>[2x]MSFTPANRAYPYTRLRRNRRDDFSRRLVRENVLTVDDLILPVFVLDGVNQRESIPSMPGVERLSIDQLLIEAEEWVALGIPALALFPVT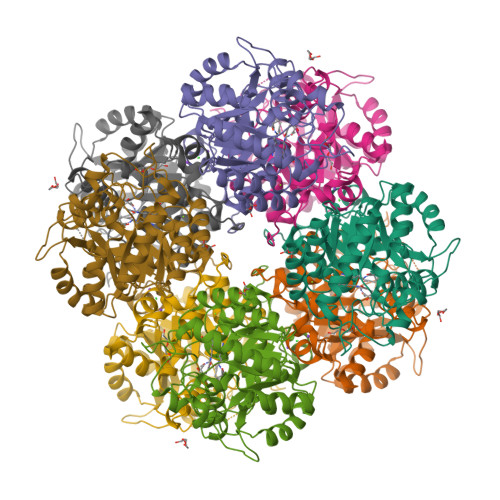PVEKKSLDAAEAYNPEGIAQRATRALRERFPELGIITDVALDPFTTHGQDGILDDDGYVLNDVSIDVLVRQALSHAEAGAQVVAPSDMMDGRIGAIREALESAGHTNVRVMAYSAKYASAYYGPFRDAVGSASNLGKGNKATYQMDPANSDEALHEVAADLAEGADMVMVKPGMPYLDIVRRVKDEFRAPTFVYQVSGEYAMHMGAIQNGWLAESVILESLTAFKRAGADGILTYFAKQAAEQLRRGR>[6x]GAMEHRAKT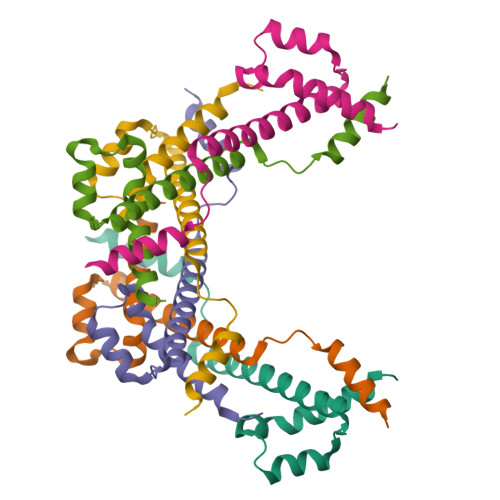KRNQELAEQLLKELPHETTSIANLVQRNNRDLDYNLEQLVRTLLQMEKEGTHVTESLINTLMETDTLTPKEQALIWPAYNLVRQMMHHAALHHI>[2x]MSTRKAVIGYYFIPTNQINNYTETDTSVVPFPVSNITPAKAKQLTHINFSFLDINSNLECAWDPATNDAKARDVVNRLTALKAHNPS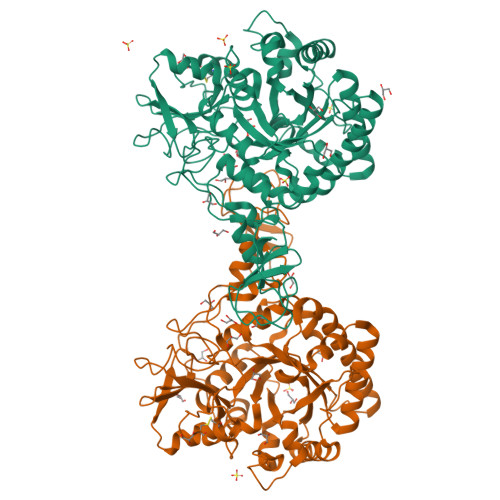LRIMFSIGGWYYSNDLGVSHANYVNAVKTPASRAKFAQSCVRIMKDYGFDGVDINWEYPQAAEVDGFIAALQEIRTLLNQQTITDGRQALPYQLTIAGAGGAFFLSRYYSKLAQIVAPLDYINLMTYDLAGPWEKVTNHQAALFGDAAGPTFYNALREANLGWSWEELTRAFPSPFSLTVDAAVQQHLMMEGVPSAKIVMGVPFYGRAFKGVSGGNGGQYSSHSTPGEDPYPSTDYWLVGCEECVRDKDPRIASYRQLEQMLQGNYGYQRLWNDKTKTPYLYHAQNGLFVTYDDAESFKYKAKYIKQQQLGGVMFWHLGQDNRNGDLLAALDRYFNAADYDDSQLDMGTGLRYTGVGPGNLPIMTAPAYVPGTTYAQGALVSYQGYVWQTKWGYITSAPGSDSAWLKVGRVA>[2x]MGSDKIHHHHHHENLYFQGRDKPLVFFNRQPSDPLTGKVDMAAMNWNDKTYYVGFDAKFGGSIQGKMILDFLASSESSVDRNGDGIIGYVLCIGDVGHNDSKVRTEGIRRALGTWTGSSDPGQAKEGQAVVGGKSYK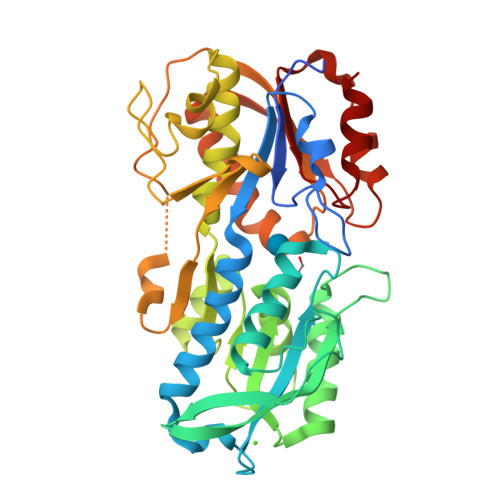VVELEGKAMTGTDGSTANTNSATESMGSWVAKFADKIDLVISNNDGMAMGCLQASNYPRGLPIFGYDANADAVESVGKGELTGTVSQNVDAQAVAVLQIIRNLLDGSSGEDVVANGISRPDAHGNKISAPVQYWEDVKAIMADNSEVTSANWKEYTRGARDAGVRQVSAPTKKVLLTVHNASNDFLASAYLPALKHYAPLLNVDLTVVQGDGQNELSCLDKFTNLDMFDAFAVNMVKTNSGADYTDKLKY> MHHHHHHSSGRENLYFQGHMETSVPPGSALVGPSCVMDDFRDPQRWKECAKQGKMPCYFDLIEENVYLTERKKNKSHRDIKRMQCE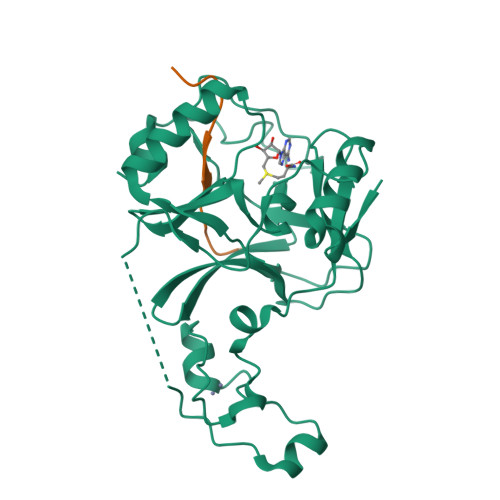CTPLSKDERAQGEIACGEDCLNRLLMIECSSRCPNGDYCSNRRFQRKQHADVEVILTEKKGWGLRAAKDLPSNTFVLEYCGEVLDHKEFKARVKEYARNKNIHYYFMALKNDEIIDATQKGNCSRFMNHSCEPNCETQKWTVNGQLRVGFFTTKLVPSGSELTFDYQFQRYGKEAQKCFCGSANCRGYLGGENRVSIRAAGGKMKKERSRK;> APATGGVMKPHRYRP> MASMTGGQQMGRGSHHHHHHENLYFQGSDKGKLSLQDVAELIRARACQRVVVMVGAGISTPSGIPDFRSPGSGLYSNLQQYDLPYPEAIFELPFFFHNPKPFFTLAKELYPGNYKPNVTHYFLRLLHDKGLLLRLYTQNIDGLERVSGIPASKLVEAHGTFASATCTVCQRPFPGEDIRADVMADRVPRCPVCTGVVKPDIVFFGEPLPQRFLLHVVDFPMADLLLILGTSLEVEPFASLTEAVRSSVP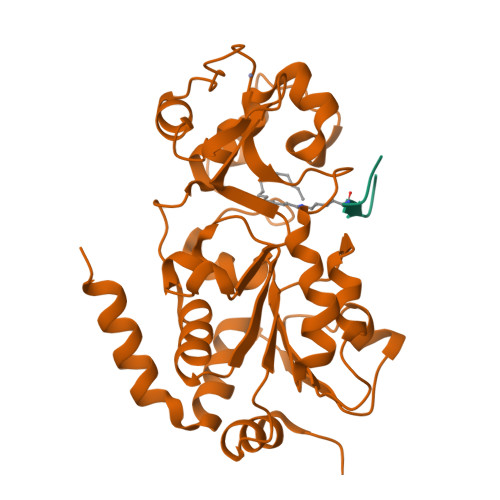RLLINRDLVGPLAWHPRSRDVAQLGDVVHGVESLVELLGWTEEMRDLVQRETGKLDGPDK;> QTARKSTGGW> MGHHHHHHHHHHSSGHIEGRHMKRIAIVGAGQSGLQLGLGLLAAGYEVTMFSNRTGEDIRRGKVMSSQCMFDTSLQIERDLGLDHWASDCPTVDGIGLAVPHPEQKGAKVIDWAARLNASAQSVDQRLKIPAWMDEFQKKGGELVFKDAGIDELEACTQSHDLTLVASGKGEISKLFERDAHKSPYDKPQRALALTYVKGMAPREPFSAVCMNLIPGVGEYAVFPALTTTGPCEIMVFEGVPGGPMDCWADVKTPEEHLARSKWILDTFTPWEAERCKDIELTDDNGILAGRFAPTVRKPVATLPSGRKVLGLADVVVLNDPITGQGSNNAAKCADTYLKSILARGDGAADAAWMQQTFDRYWFGYAQWVTQWTNMLLAPPPPHVLNLLGSAGAVPPLASAF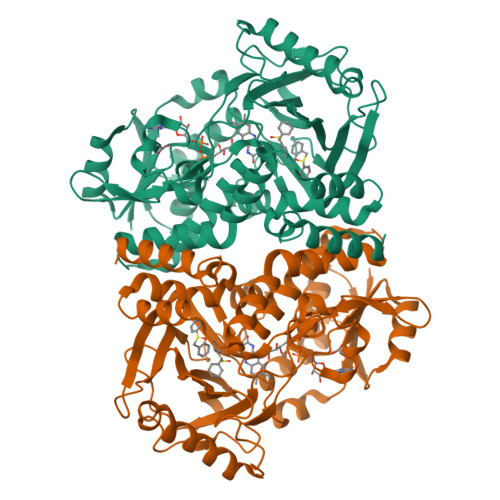ANGFDDPRTFFPWFADAAESERYIATCAAVA> MSLLDRGGTYGSPEDGFDPVTVYPEVTRK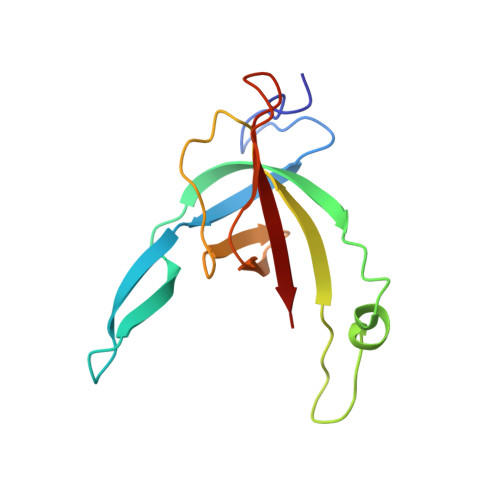DRLGNTLVGPSLTGIETVARFQVQGQSGTSARRAEMDDIGDMTEQVYTMRLPRSFTTELKSGSEVVWRGERWGVYGEPRRYKGSRRIAHLEYTVRRF4-[2-[5-(dimethylamino)pentylamino]-8-[[(2~{S})-1-oxidanylpropan-2-yl]amino]quinazolin-6-yl]-5-ethyl-2-fluoranyl-phenol 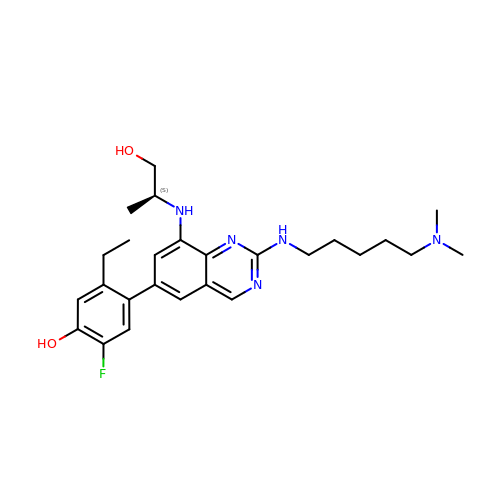| C26 H36 F N5 O2 | XUZGLJHOFPPBEF-KRWDZBQOSA-N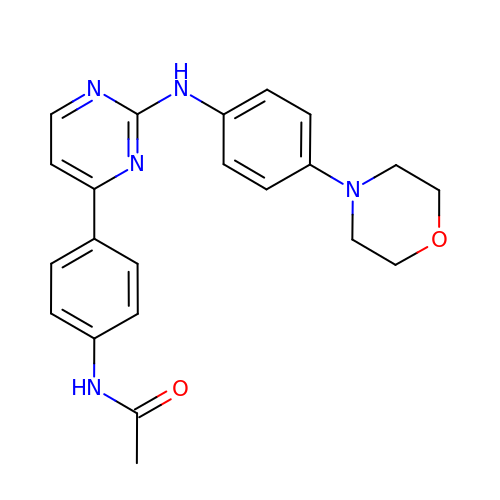N-[4-[2-[(4-morpholin-4-ylphenyl)amino]pyrimidin-4-yl]phenyl]ethanamide | C22 H23 N5 O2 | RMBHIVQOFNFWFU-UHFFFAOYSA-N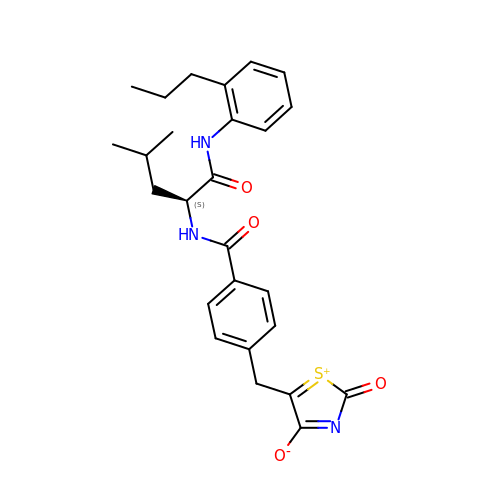5-[[4-[[(2~{S})-4-methyl-1-oxidanylidene-1-[(2-propylphenyl)amino]pentan-2-yl]carbamoyl]phenyl]methyl]-2-oxidanylidene-1,3-thiazol-1-ium-4-olate | C26 H29 N3 O4 S | NWLPQCZZJXMUOM-NRFANRHFSA-N>MYEMPKLPYANNALEPVISQQTIDYHYGKHLQTYVNNLNSLVPGTEYEGKTVEAIVASAPDGAIFNNAGQVLNHTLYFLQFAPKPAKNEPAGKLGEAIKRDFGSFENFKKEFNAASVGLFGSGWAWLSVDKDGKLHITKEPNGSNPVRAGLKPLLGFDVWEHAYYLDYQNRRADHVNKLWEIIDWDVVEKRL[8x]

Here we studied metal-preference evolution within the natural diversity of the iron/manganese superoxide dismutase (SodFM) family of reactive oxygen species scavengers. Only a few metalloenzymes have been rigorously demonstrated to be cambialistic in vivo, including some iron (Fe)- or manganese (Mn)-dependent superoxide dismutases (SODs; SodFMs); metalloenzymes that play an important role in cellular reactive oxygen species defence. To study this process, we leveraged the existence of naturally Fe-specific, Mn-specific and flexible Fe/Mn-cambialistic SodFM homologues, which differentially utilize these metals to catalyse the detoxification of superoxide. By combining phylogenetics, biochemistry and structural biology, we demonstrate that SodFM metal utilization can be evolutionarily fine tuned by sliding along a scale between perfect manganese and iron specificities.

More cambialistic outliers included the Bacteroides fragilis (aCR 0.98) and Coprobacter fastidiosus (aCR 0.99) SodFM2s, which seem to have evolved higher Mn activity from their most likely Fe-preferring ancestor. This confirmed that the presence of GD-2 and AD-2 within the context of otherwise predominantly Fe-preferring SodFMs can indicate potential evolutionary metal-preference modulation events. We identified at least two independent emergences of cambialism in this group, once from Fe-SodFM2 and a second time from Mn-SodFM1 ancestors. Next, we leveraged the cambialistic SODs from S. aureus and B. fragilis to investigate the specific role of the XD-2 position in determining metal preference. Therefore, our results suggest that the S. aureus cambialistic SodFM1 has potential for evolution towards higher Fe preference, whereas the B. fragilis cambialistic SodFM2 has reached the highest possible level of Mn preference via mutagenesis of the XD-2 residue alone. Importantly, consistent with previous reports, comparison of four protein crystal structures of the WT and mutant SodFMs we determined here indicated that metal-preference modulation by XD-2 and Q/H occurs without any significant changes to the secondary metal coordination sphere within the resolution limits of the solved structures.> MATYSLANERLRALEDIEREIGAILQNAGTVILELSKEKTNERLLDRQAAAFTASVQHVEAE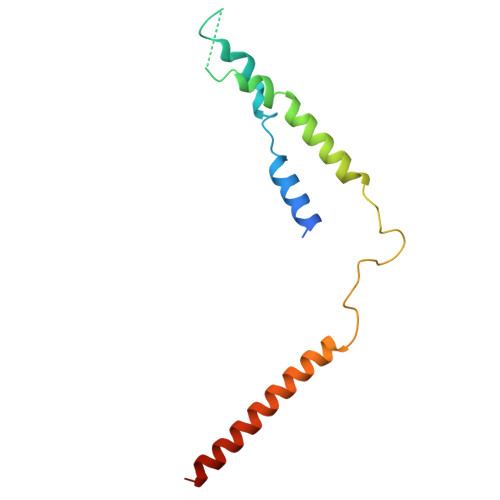LSAQIRYLTQVATGQPHEGSSYSSRKDCQMALKRVDYARLKLSDVARTCEQMLEN> MGSSHHHHHHSSGPQQGLRQQKLVEVAKGYSCTSVNTTIFRNNSLVTHGDEQYISYYDADGYLVLGKRKLNSKQWTLHRTQYRGNVKDAHNIISIMVDGEGYLHVSFDHHGHKLNYCRSIAPGSLELGDKMPMTGVDEGNVTYPEFYPLTDGDLLFVYRSGSSGRGNLVMNRYSLKDHKWARVQDVLIDGEDKRNAYWQLYVDEKGTIHLSWVWRETWQVETNHDLCYARSFDNGVTWYKSDGEQYKLPITASNAEYACRIPQNSELINQTSMSADAGGNPYIATYWRSSDSEVPQYRIVWNDGKTWHNRQVTDRKTPFTLKGGGTKMIPVARPRIVVEDGEIFYIFRDEERGSRVSMAHTADVANGKWIVTDLTDFSVDAWEPSHDTELWKKQRKLNLFVQHTCQGDGERTAEI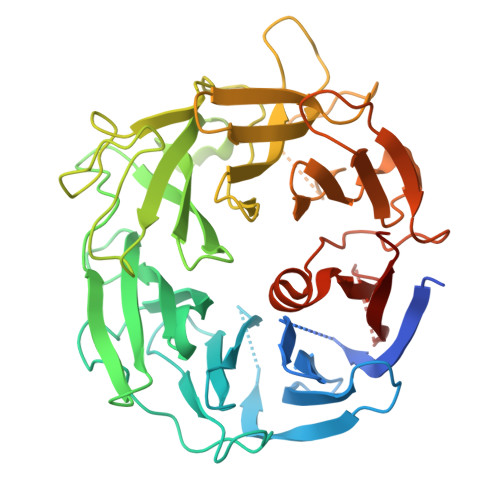EPQMIYVLEANTNTKK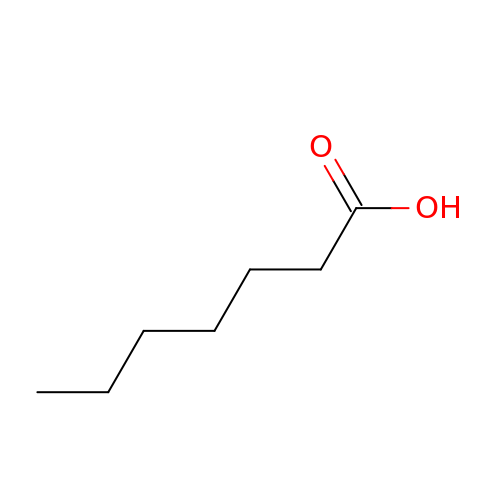HEPTANOIC ACID | C7 H14 O2 | MNWFXJYAOYHMED-UHFFFAOYSA-N>[2x]GRVYLVGAGPGDPELLTLKAYRLLKEAPVVLYDRLVDERVLALAPGEKVYVGKEEGESEKQEEIHRLLLRHARAHPFVVRLKGGDPMV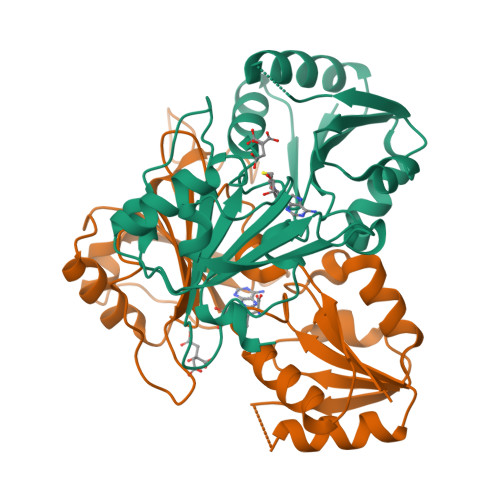FGRGGEEVLFLLRHGVPVEVVPGVTSLLASGLPLTHRGLAHGFAAVSGVLEGGGYPDLRPFARVPTLVVLMGVGRRVWIAKELLRLGRDPREPTLFVERASTPKERRVHARLEEVAEGKVEVRPPALWILGEVVRVFAEKEAPVDALALGG Transcription activator-like (TAL) effectors specifically bind to double stranded (ds) DNA through a central domain of tandem repeats. Each TAL effector (TALE) repeat comprises 33–35 amino acids and recognizes one specific DNA base through a highly variable residue at a fixed position in the repeat. The crystal structures of TAL effector (TALE) proteins bound to their respective target DNAs have revealed that the residue at position 13 is the only one directly involved in DNA base recognition, whereas the 12th residue stabilizes the proper loop conformation. dHax3, an engineered TALE protein, proved to be a useful scaffold for structural characterizations. We then present fifteen crystal structures of engineered dHax3 variants in complex with target DNA molecules, which elucidate the structural basis for the recognition of bases adenine (A) and guanine (G) by reported or uncharacterized TALE codes.

As a proof-of-principle, we generated two dHax3 variants, dHax3-NI, in which Ile34 was introduced at repeat 7 to replace Ser34 for recognition of base A, and dTALE (standing for designed TALE repeats), in which the RVDs in repeats 3–12 were replaced and the protein recognize an artificial DNA element (5′-TCCAACTACTAGA-3′). Two structures were determined for DNA-bound dHax3-NI at 2.8 Å and 2.2 Å, respectively. During structural analysis of DNA-bound dHax3-NI, we found that while the low-resolution structure (2.8 Å) can be completely overlaid with those of dHax3 and dTALE, the high-resolution one (2.2 Å) deviates considerably from all the other DNA-bound TALE structures. In contrast, the structural difference between the high-resolution structure of DNA-bound dHax3-NI and the other DNA-bound TALE structures is a combination of both axial compression and rotational tightening of the TALE repeats accompanied by a slight distortion of the DNA duplex. The overall conformational change of the complex indicates that TALE repeats may retain structural flexibility even after binding to DNA. Despite the prominent conformational changes between the overall structures, when the individual repeats of the high and low-resolution structures of DNA-bound dHax3-NI are superimposed, the RMSD value is 0.23 Å over 30 Cα atoms of the second repeat. Similar to the comparison between DNA-free and DNA-bound dHax3 structures, the overall changes result from the accumulative effect of small alterations in the φ and ϕ values of the peptide bonds of residues 14–22 (corresponding to the previously designated residues 26–34) in each repeat. Supporting this notion, the 22 repeats from both the high and low-resolution structures of dHax3-NI can be precisely superimposed with the pairwise RMSD values between 0.3–0.6 Å over 29 to 33 Cα atoms, with the deviations mainly at the segment containing residues 13–22 in each repeat. These structural observations suggest that the residues 13–22 within a TALE repeat are responsible for the structural plasticity of the repeat.

>[2x]MQWSGARALEALLTVAGELRGPPLQLDTGQLLKIAKRGGVTAVEAVHAWRNALTGAPLNLTPEQVVAIASHDGGKQALETVQRLLPVLCQAHGLTPQQVVAIASHDGGKQALETVQRLLPVLCQAHGLTPEQVVAIASHDGGKQALETVQALLPVLCQAHGLTPEQVVAIASNGGGKQALETVQRLLPVLCQAHGLTPQQVVAIASNGGGKQALETVQRLLPVLCQAHGLTPQQVVAIASNGGGKQALETVQRLLPVLCQAHGLTPQQVVAIASNIGGKQALETVQRLLPVLCQAHGLTPQQVVAIASNGGGKQALETVQRLLPVLCQAHGLTPQQVVAIASHDGGKQALETVQRLLPVLCQAHGLTPEQVVAIASNGGGKQALETVQRLLPVLCQAHGLTPEQVVAIASHDGGKQALETVQRLLPVLCQAHGLTPQQVVAIASNGGGRPALESIVAQLSRPDPALAALTNDHLVALACLGGRPALDAVKKLEHHHHHH We present a new class of ArMs featuring a genetically encoded noble‐metal‐binding site based on a non‐canonical thiophenol‐based amino acid, 4‐mercaptophenylalanine (pSHF), incorporated in the transcriptional regulator LmrR through stop codon suppression. Next, we investigated the incorporation of pSHF into Lactococcal multidrug resistance regulator (LmrR), which has been demonstrated to be a highly versatile protein scaffold for artificial enzyme design. We selected position V15 for incorporation, since this places pSHF inside the hydrophobic pocket at the dimer interface. Here, we report a new class of artificial metalloenzymes featuring a genetically encoded thiophenol for binding noble metals and the application of this design approach by the creation of an artificial gold enzyme that shows efficient catalysis of abiological hydroamination reactions.

Optimisation of the expression temperature, as well as the addition of the reductant tris(2‐carboxyethyl)phosphine (TCEP) during protein production and purification, minimised modifications of the thiol group. Using the optimised protocol, after affinity chromatography purification, LmrR_V15pSHF was obtained in yields of 75–145 mg/L cell culture. LmrR_V15pSHF is envisioned to have two specific metal‐binding sites per dimer. To our delight, LmrR_V15pSHF binds a variety of noble metals, albeit with varying degrees of efficiency and sometimes accompanied by oxidation. In most cases, there was substantially more of the metal adduct detectable for LmrR_V15pSHF compared to LmrR_WT and LmrR_V15C, showing the potency of pSHF in binding noble‐metal ions or complexes.

>[2x]MAEIPKEMLRAQTNAILLNVLKQGDNYVYGIIKQVKEASNGEMELNEATLYTIFKRLEKDGIISSYWGDESQGGRRKYYRLTEIGHENMRLAFESWSRVDKIIENLEANKKSEAIKSRWSHPQFEK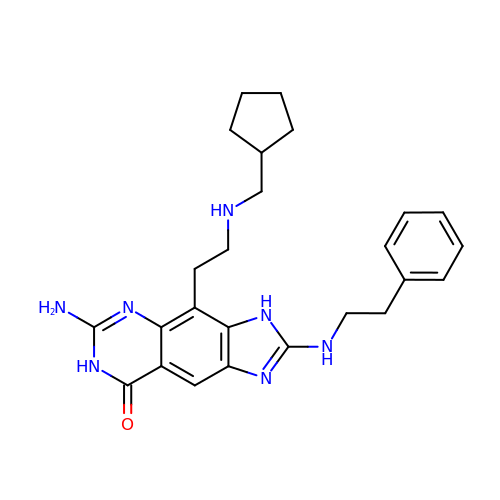6-amino-4-{2-[(cyclopentylmethyl)amino]ethyl}-2-[(2-phenylethyl)amino]-3,7-dihydro-8H-imidazo[4,5-g]quinazolin-8-one | C25 H31 N7 O | RDFXKIVPJRMHKW-UHFFFAOYSA-N VCCN1 was recently identified as a voltage-gated chloride channel residing in the thylakoid membrane, where it plays a key role in photoreaction tuning to avoid the generation of reactive oxygen species (ROS). VCCN1 structurally resembles its animal homolog, bestrophin, a Ca2+-gated anion channel. However, unlike bestrophin channels, VCCN1 lacks the Ca2+-binding motif but instead contains an N-terminal charged helix that is anchored to the lipid membrane through an additional amphipathic helix. MdVCCN1 forms a symmetric homopentamer, with each subunit consisting of three domains: transmembrane domain (TMD), N-terminal domain (NTD), and stromal domain (SMD).

By the structural analogy, we assumed that the conformational change of the Tyr332 residue triggers MdVCCN1 gating via the hydrogen bond interaction, and that the Y332A mutation may mimic the state after the conformational change. Accordingly, to test our hypothesis, we determined the structure of the MdVCCN1 Y332A mutant reconstituted in nanodiscs by cryo-EM. The overall assembly and subunit folding of the Y332A mutant are quite similar to those of the WT structure in nanodiscs, with RMSD values below 0.36 Å for 335 Cα atoms, demonstrating that the Y332A mutation does not affect the overall structural integrity. In the mutant structure, however, the Glu195 residue flips toward the central axis, and the Phe192 residue in the neck flips away from the central axis and resides in the space occupied by Tyr332 in the WT structure. Consequently, Glu195 is directly exposed to the ion permeation pathway, and thus may affect the anion permeability. Notably, this local conformational change of the Phe residue was similarly observed in the open structure of GgBEST120, while the other neck residues remained in the closed conformation. Consistently, the pore radius of the Y332A mutant was widened only at the position of Phe192. Thus, the Y332A mutant seems to mimic the ‘partially opened’ state of VCCN1, whereas the whole neck opening requires larger movements, triggered by the conformational change of Tyr332. However, the Y332F mutant exhibited greatly reduced whole-cell currents, whereas the Y332A mutant showed only slightly reduced currents. Taken together, these electrophysiological and structural analyses demonstrated that the inter-helical interactions near the neck region are important for channel activity in the VCCN1 family.

> MPNPSPPSSSSPVQTLISILRIIPDWSDRTQERGMRQHRTLYDHEKWMHHRSSYRHLRHLLSSLSSRVILSLIPPVIAFTLVAVVIASYNTAVALDLLPGIFPLLRSSSLPYQLTAPALALLLVFRTEASYSRFEEGRKSWTEVIAGANDFARQIISSVETSGDAQLKKALLQYIVAFPVALKCHVIYGSDIARDLQNLLEVDDLLVVLNSKHRPGCIIQFISRSLQLLKLEESRRIMLQSKISCFHEGIGICEQLIGTPIPLSATRLTSRFLVLWHLTLPIILWDDCHWIVVPATFISAASLFCIEQVGVLIEEPFPMLALDDLCNSVRNNVQEALASEKLIRARLAAKGRIQSEQQFQNGQPRPENLYFQ>[4x]SNANNLFVY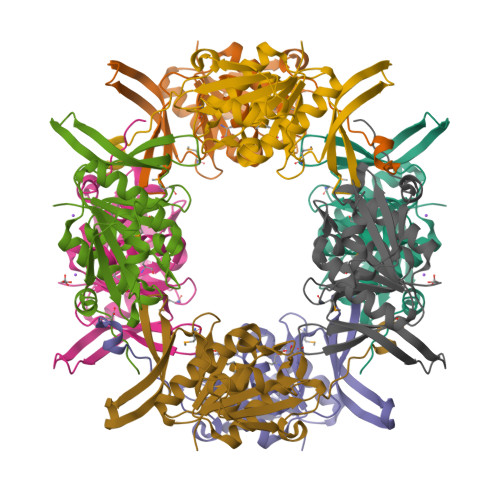CEIEEGIVADVSLELLTKGRSLANELNCQLEAVVAGTGLKEIEKQILPYGVDKLHVFDAEGLYPYTSLPHTSILVNLFKEEQPQICLMGATVIGRDLGPRVSSALTSGLTADCTSLEIGDHEDKKEGKVYKNLLYQIRPAFGGNIVATIVNPEHRPQMATVREGVMKKEIVSPAYQGEVIRHDVKKYVADTDYVVKVIERHVEKAKNN> XDS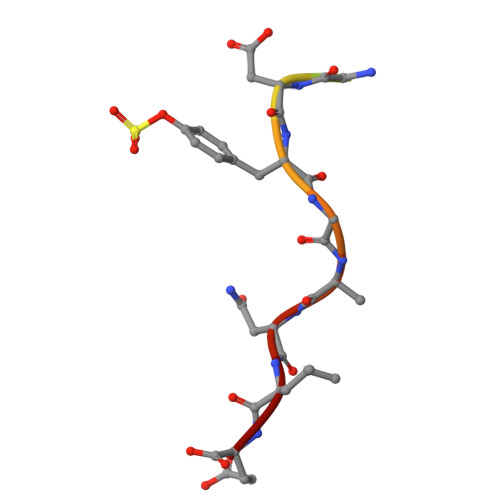FPDGDYGANLE>GSHMYVIVVYDVNVERVNRVHKLLKT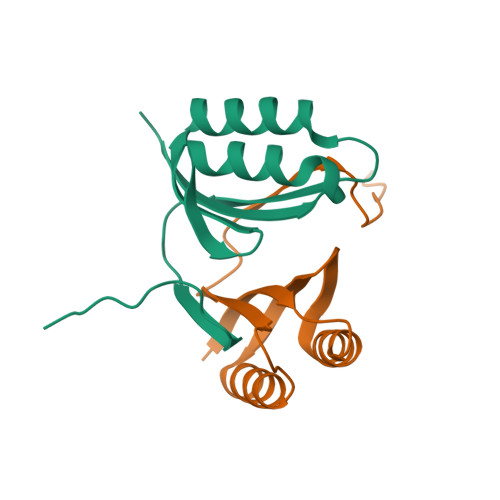YLFWRQNSVFEGELSKAQLYELEMRLKRIVKEDDSVLIYIFPGKNFDLHVVGRDKSPVEMII[2x]>MVNNNRPRRQRAQRVVVTTTQTAPVPQQNVPRNGRRRRNRTRRNRRRVRGMNMAALTRLSQPGLAFLKCAFAPPDFNTDPGKGIPDRFEGKVVSRKDVLNQSISFTAGQDTFILIAPTPGVAYWSASVPAGTFPTSATTFNPVNYPGFTSMFGTTSTSRSDQVSSFRYASMNVGIYPTSNLMQFAGSITVWKCPVKLSTVQFPVATDPATSSLVHTLVGLDGVLAVGPDNFSESFIKGVFSQSACNEPDFEFNDILEGIQTLPPANVSLGSTGQPFTMDSGAEATSGVVGWGNMDTIVIRVSAPEGAVNSAILKAWSCI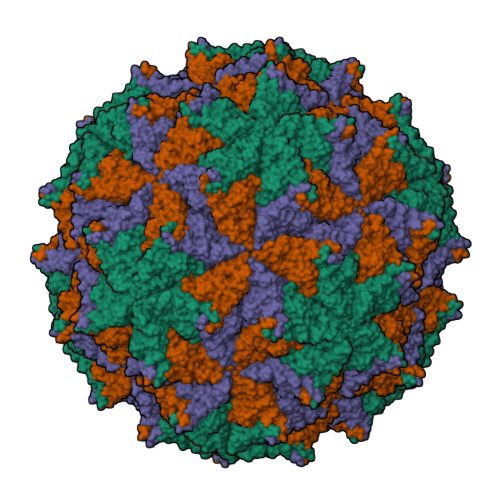EYRPNPNAMLYQFGHDSPPLDEVALQEYRTVARSLPVAVIAAQN[3x];>[3x]ASMWERVKSIIKSSLAAASNIPGPIGVAASGISGLSALFEGFGF>MRRSQRADGLAAVLAIGTANPPNCVTQEEIPDFYFRVTNSDHLTALKDKFKRICQEMGVQRRYLHHTEEMLSAHPEFVDRDAPSLDARLDIAADAVPELAAEAAKKAIAEWGRPAADITHLVVTTNSGAHVPGVDFRLVPLLGLRPSVRRTMLHLNGCFAGCAALRLAKDLAENSRGARVLVVAAELTLMYFTGPDEGCFRTLLVQGLFGDGAAAVIVGADADDVERPLFEIVSAAQTIIPESDHALNMRFTERRLDGVLGRQVPGLIGDNVERCLLDMFGPLLGGDGGGGWNDLFWAVHPGSSTIMDQVDAALGLEPGKL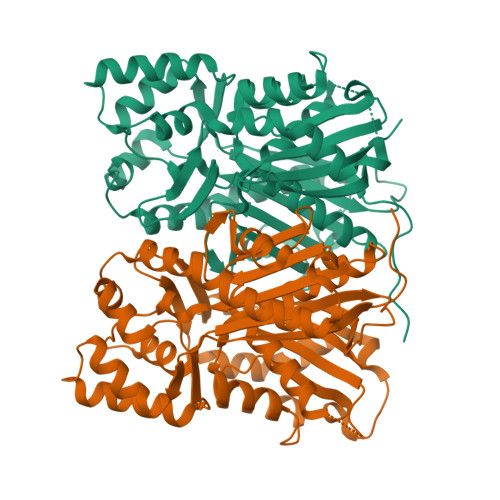AASRRVLSDYGNMSGATVIFALDELRRQRKEAAAAGEWPELGVMMAFGPGMTVDAMLLHATSHHHH[2x]(2R,3R,4R,5S,6R)-5-fluoranyl-6-(hydroxymethyl)oxane-2,3,4-triol | 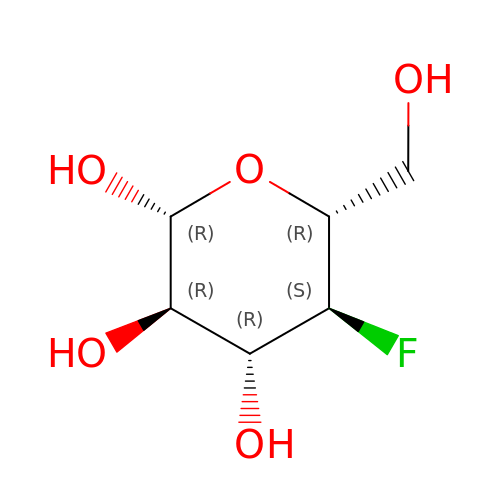C6 H11 F O5 | FIHYONSINSKFAH-VFUOTHLCSA-N> MTKVDFWPTLKDAYEPLYPQQLEILRQQVV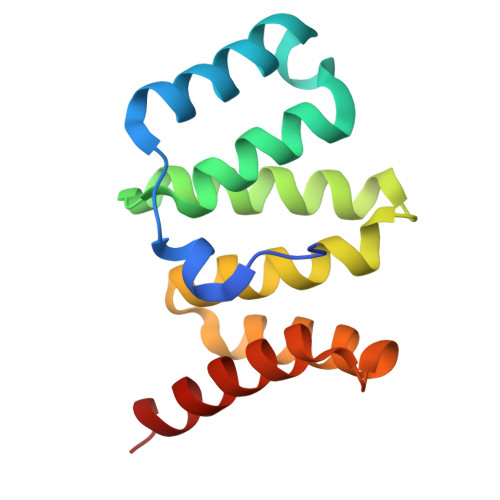SEGGPTATIQSRFNYAWGLIKSTDVNDERLGVKILTDIYKEAESRRRECLYYLTIGCYKLGEYSMAKRYVDTLFEHERNNKQVGALKSMVEDKIQKETL> ETGCPANCLCSKTDINCKKPDDGNLFPLLEGQDSGSSNGQTSIQITDISRNITSIHIENWKNLQTLNAVDMELYTGLQRLTIRNSGLRNIQPRAFAKNPHLRYIDLSGNRLTTLSWQLFQTLRLFDLRLERNPFQCSCDIRWIQLWQEKGEA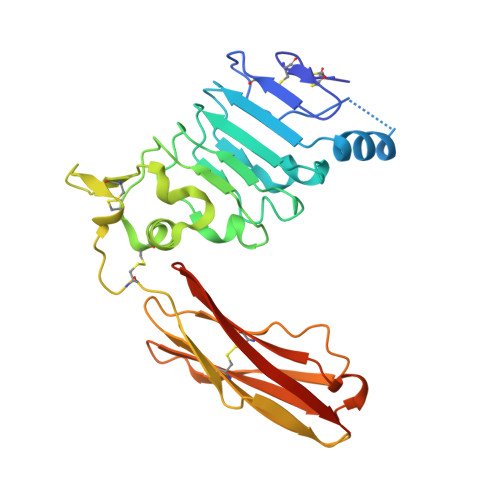NLQSQQLHCMNLDTAVILLRNMNITQCDLPEISVSHVNLTVREGENAVITCQGSGSPLPDVDWTVADLHSINTHQTNLQWTNVHAIQLTLVNVTSEDNGFLLTCIAENVVGMSQASVLLTVYGTKHHHHHH>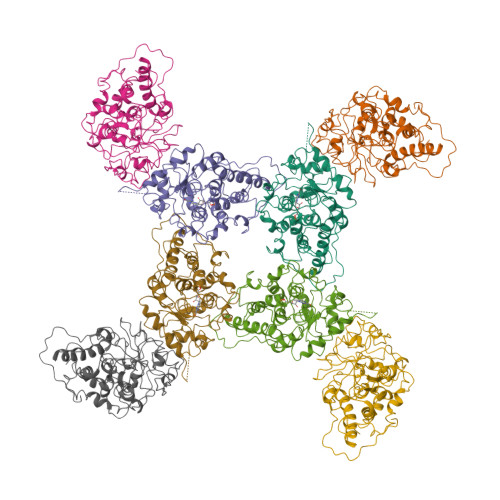[2x]MEITNVNEYEAIAKQKLPKMVYDFYASGAEDQWTLAENRNAFSRILFRPRILIDVTNIDMTTTILGFKISMPIMIAPTAMQKMAHPEGEYATARAASAAGTIMTLSSWATSSVEEVASTGPGIRFFQLYVYKDRNVVAQLVRRAERAGFKAIALTVDTPRLGRREADIKNRFVLPPFLTLKNFEGIDLGKMDKANDSGLSSYVAGQIDRSLSWKDVAWLQTITSLPILVKGVITAEDARLAVQHGAAGIIVSNHGARQLDYVPATIMALEEVVKAAQGRIPVFLDGGVRRGTDVFKALALGAAGVFIGRPVVFSLAAEGEAGVKKVLQMMRDEFELTMALSGCRSLKEISRSHIAADWDGPSSRAVARL> MDSNTVSSFQVDCFLWHVRKQVVDQELG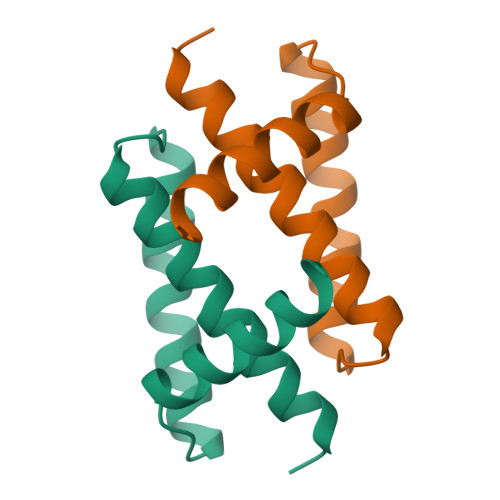DAPFLDRLRRDQKSLRGRGSTLGLNIEAATHVGKQIVEKILKEED>[4x]MAPHGDGLSDIEEPEVDAQSEILRPISSVVFVIAMQAEALPLVNKFGLSETTDSPLGKGLPWVLYHGVHKDLRINVVCPGRDAALGIDSVGTVPASLITFASIQALKPDIIINAGTCGGFKVKGANIGDVFLVSDVVFHDRRIPIPMFDLYGVGLRQAFSTPNLLKELNLKIG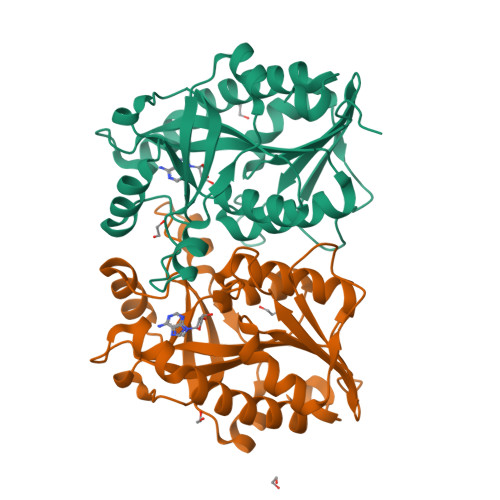RLSTGDSLDMSTQDETLIIANDATLKDMEGAAVAYVADLLKIPVVFLKAVTDLVDGDKPTAEEFLQNLTVVTAALEGTATKVINFINGRNLSDL>[2x]SAPILIQGAMDVEVETLVAALKDKQELTVGSWTYWQGTLSGY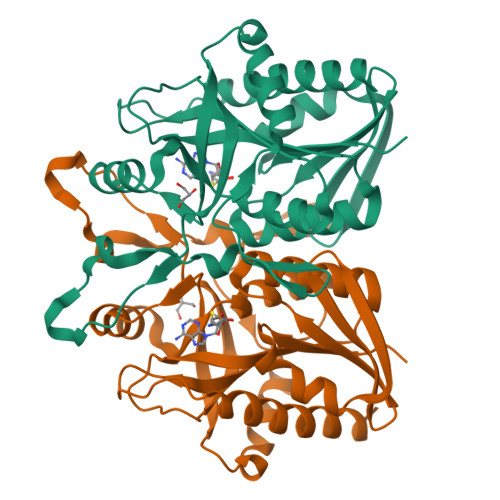PVVVSRTEVGLANAAAATTLAMERFQPRLVINQGTAGGHDPALHRGDIVIGTKSFNMGAYRSDLTPAEQGVDPSKWHNFEVTMRLRDNGKLVEHSSFAGDPELVGRALGMADRYRHGRVVPGIIGTADEWNRQVARINWLHQTYQTAAEEMETSSAALVAEAYKVPFVGIRVLSNTDLHGEEFDPQTAIHCQQFVIDYAKALINGF> EDMPVERILEAELAVEPKTETYVEANMGLNPSSPNDPVTNICQAADKQLFTLVEWAKRIPHFSELPLDDQVILLRAGWNELLIASFSHRSIAVKDGILLATGL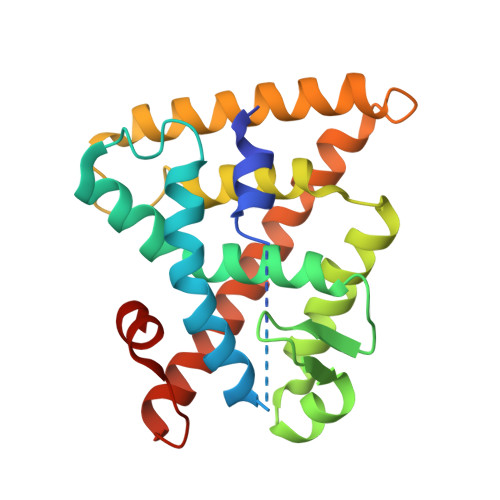HVHRNSAHSAGVGAIFDRVLTELVSKMRDMQMDKTELGCLRAIVLFNPDSKGLSNPAEVEALREKVYASLEAYCKHKYPEQPGRFAKLLLRLPALRSIGLKCLEHLFFFKLIGDTPIDTFLMEMLEAP6-[(2-methoxybenzyl)amino]pyridine-3-carboxamide | C14 H15 N3 O2 | 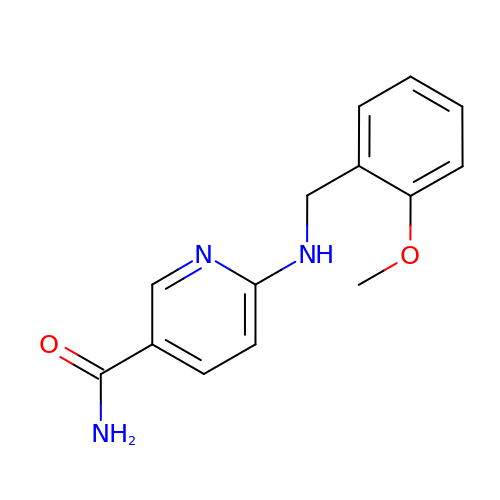OZFDPNFXJQTLGG-UHFFFAOYSA-N>[2x]NECLGTIGPVTPLDASDFALDIRMPGVTPKESDTYFCMSMRLPVDEEAFVIDFK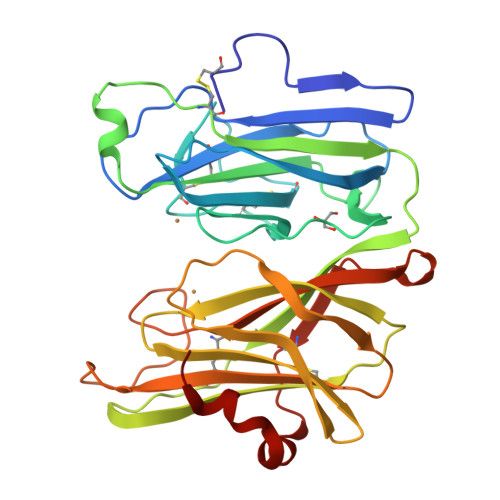PRASMDTVHHMLLFGCNMPSSTGSYWFCDEGTCTDKANILYAWARNAPPTRLPKGVGFRVGGETGSKYFVLQVHYGDISAFRDNHKDCSGVSVHLTRVPQPLIAGMYLMMSVDTVIPPGEKVVNADISCQYKMYPMHVFAYRVHTHHLGKVVSGYRVRNGQWTLIGRQNPQLPEAFYPVEHPVDVTFGDILAARCVFTGEGRTEATHIGGTSSDEMCNLYIMYYMEAKYALSFMTCTKNVAPDMFRTIPAEANIPI> MSEYMDDVDREFINCLFPSYLLQQPVAYDLWILYLQHRKLFHKLKNTNLINADENPTGVGMGRTKLTALTRKEIWSKLMNLGVLGTISFEAVNDDYLIQVYKYFYPDVNDFTLRFGVKDSNKNSVRVMKASSDMRKNAQELLEPVLSEREMALNSNTSLENDRNDDDDDDDDDDDDDDDDDDDDDESDLESLEGEVDTDTDDNNEGDGSDNHEEGGEEGSRGADADVSSAQQRAERVADPWIYQRSRSAINIETESRNLWDTSDKNSGLQYYPPDQSPSSSFSSPRVSSGNDKNDNEATNVLSNSGSKKKNSMIPDIYKILGYFLPSRWQAQPNNSLQLSQDGITHLQPNPDYHSYMTYERSSASSASTRNRLRTSFENSGKVDFAVTWANKSLPDNKLTIFYYEIKVLSVTSTESAENSNIVIGYKLVENELMEATTKKSVSRSSVAGSSSSLGGSNNMSSNRVPSTSFTMEGTQRRDYIYEGGVSAMSLNVDGSINKCQKYGFDLNVFGYCG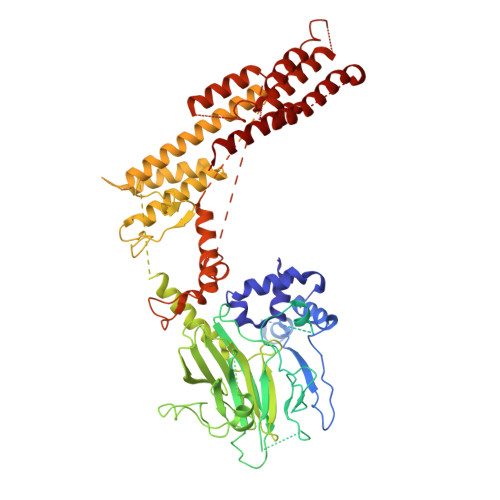FDGLITNSTEQSKEYAKPFGRDDVIGCGINFIDGSIFFTKNGIHLGNAFTDLNDLEFVPYVALRPGNSIKTNFGLNEDFVFDIIGYQDKWKSLAYEHICRGRQMDVSIEEFDSDESEEDETENGPEENKSTNVNEDLMDIDQEDGAAGNKDTKKLNDEKDNNLKFLLGEDNRFIDGKLVRPDVNNINNLSVDDGSLPNTLNVMINDYLIHEGLVDVAKGFLKDLQKDAVNVNGQHSESKDVIRHNERQIMKEERMVKIRQELRYLINKGQISKCINYIDNEIPDLLKNNLELVFELKLANYLVMIKKSSSKDDDEIENLILKGQELSNEFIYDTKIPQSLRDRFSGQLSNVSALLAYSNPLVEAPKEISGYLSDEYLQERLFQVSNNTILTFLHKDSECALENVISNTRAMLSTLLEYNAFGSTNSSDPRYYKAINFDEDVLNLXXXXXXXXXXXXXXXXXXXXXXXXXXXXXXXXXXXXXXXXXXXXXXXXXXXXXXXXXXXXXXXXXXXXXXXXXXXXXXXXXXXXXXXXXXXXXXXXXXXXXXXXXX N-succinyl-L-phenylglycine | C12 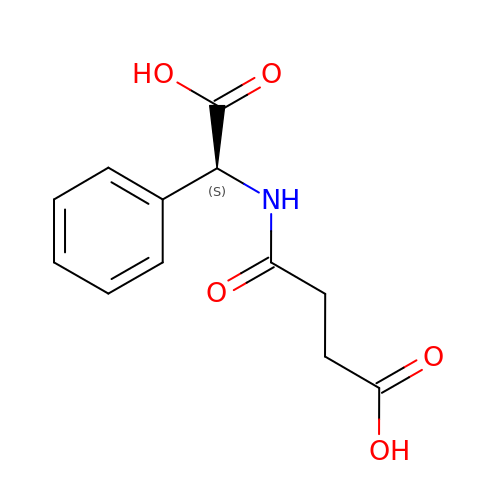H13 N O5 | GQFHIYFXQQEWME-NSHDSACASA-N> GPLGSIAQARRQYHFESNQRTCNMTVLSMLPTLREALMQQLNSESLTALLKNRPSNK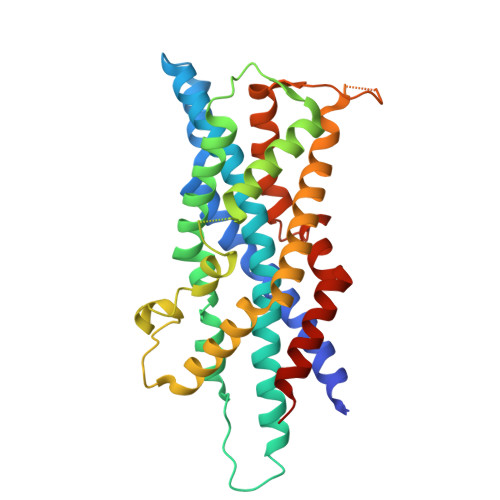LEIWEDLKIISFTRSTVAVYSTCMLVVLLRVQLNIIGGYIYLDNAAVGKNGTTILAPPDVQQQYLSSIQHLLGDGLTELITVIKQAVQKVLGSVSLKHSLSLLDLEQKLKEIRNLVEQHKSSSWINKDGSKPLLCHYMMPDEETPLAVQACGLSPRDITTIKLLNETRDMLESPDFSTVLNTCLNRGFSRLLDNMAEFFRPTEQDLQHGNSMNSLSSVSLPLAKIIPIVNGQIHSVCSETPSHFVQDLLTMEQVKDFAANVYEAFSTPQQLEK> MGSSHHHHHHSSGRENLYFQGHMNHSIPTLRTERLTLRPLAMADFPAYRDFMASPRSTGVGGPYDLPSTWGVFCHDLANWHFFGHGALMIDLGETGECI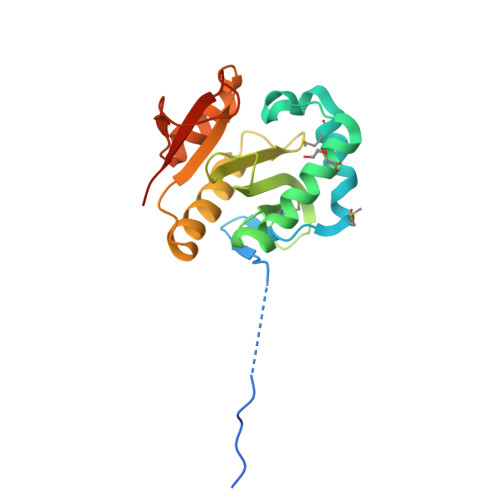GQIGINHGPLFPEKELGWLLYEGHEGRGYAAEAAVALRDWAFETLNLPTLVSYVSPQNRKSAAVAERIGGTLDPLAPRSDPEDLVYRYHQVKTAGS> SEEPPFDIRALRADIEDMISEKLELGPSLIRLAWHEAASYDCFKKDGSPNSASMRFKPECLYAGNKGLDIPRKALETLKKKYPQISYADLWVLAAYVAIEYMGGPTIPFCWGRVDAKDGSVCGPDGRLP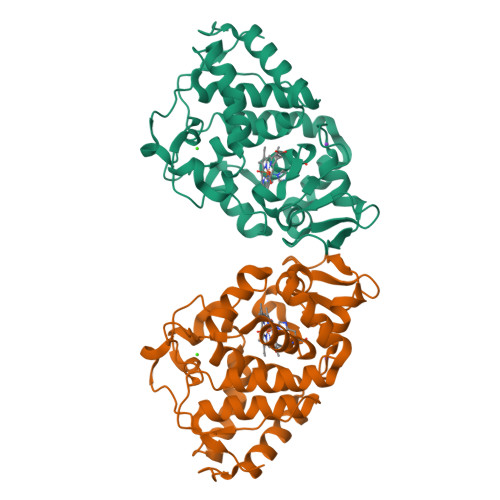DGSKTQSHVREVFRRLGFNDQETVALIGAHTCGECHIEFSGYHGPWTHRKNGFDNSFFTQLLDEDWVLNPKVEQMQLMDRATTKLMMLPSDVCLLLDPSYRKYVELYAKDNDRFNKDFANAFKKLTELGTRNLHKAPASES>[3x]MGSSHHHHHHSQDPENLYFQGTGKFRYMPFSPAGTPFGFTDRRYLTMNEVGYVSTVKNSEQYSITVSFFDVGRFREYHFEDLFGYDLCFLNEKGTLFGQSKTGQIQYRPHDSIHSNWTKIIPLQAGERITSVAAT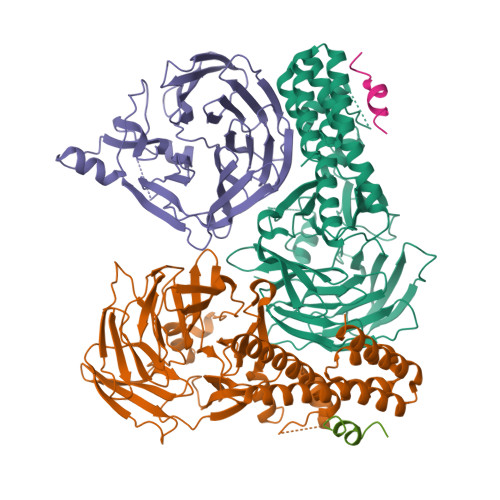PVRVIVGTSLGYFRSFNQFGVPFAVEKTSPIVALTAQNYRVFSVHYSQFHGLSYSLSELGTSSKRYYKRECPLPMSLPNINSDMKKDANLDYYNFNPMGIKSLFFSSYGDPCIFGSDNTLLLLSKWRSPEESKWLPILDSNMEIWKMSGGKETTDIHVWPLALAYDTLNCILVKGKHIWPEFPLPLPSEMEIRMPVFVKSKLLEENKAILNKKNEIGADTEAEEGEEDKEIQIPVSMAAEEEYLRSKVLSELLTDTLENDGEMYGNENEVLAALNGAYDKALLRLFASACSDQNVEKALSLAHELKQDRALTAAVKISERAELPSLVKKINNIREARYEQQLK;>[2x]SLRNIDDILDDIEGDLT3-(3-{3-[(2,4-diamino-6-ethylpyrimidin-5-yl)oxy]propoxy}phenyl)propanoic acid | C18 H24 N4 O4 | 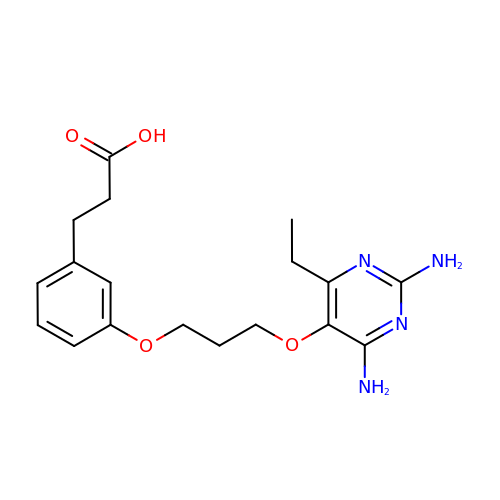HMQJRDLOETYJSB-UHFFFAOYSA-N>MSSAIKEVQGAPVKWVTNWTPEAIRGLVDQEKGLLD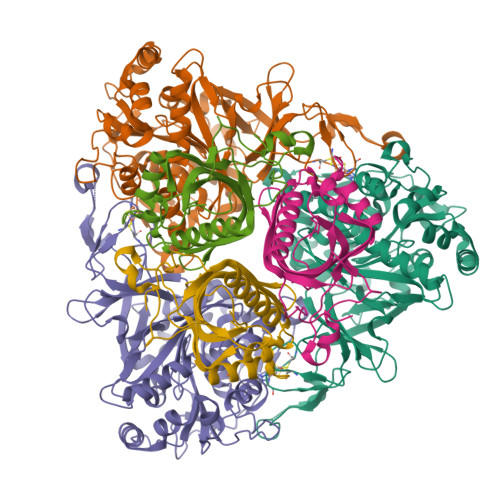PRIYADQSLYELELERVFGRSWLLLGHESHVPETGDFLATYMGEDPVVMVRQKDKSIKVFLNQCRHRGMRICRSDAGNAKAFTCSYHGWAYDIAGKLVNVPFEKEAFCDKKEGDCGFDKAEWGPLQARVATYKGLVFANWDVQAPDLETYLGDARPYMDVMLDRTPAGTVAIGGMQKWVIPCNWKFAAEQFCSDMYHAGTTTHLSGILAGIPPEMDLSQAQIPTKGNQFRAAWGGHGSGWYVDEPGSLLAVMGPKVTQYWTEGPAAELAEQRLGHTGMPVRRMVGQHMTIFPTCSFLPGINTIRTWHPRGPNEIEVWAFTLVDADAPAEIKEEYRRHNIRNFSAGGVFEQDDGENWVEIQKGLRGYKAKSQPLNAQMGLGRSQTGHPDFPGNVGYVYAEEAARGMYHHWMRMMSEPSWATLKP[4x];>[4x]MTNPSPHFFKTFEWPSKAAGLELQNEIEQFYYREAQLLDHRAYEAWFALLDKDIHYFMPLRTNRMIREGELEYSGDQDLAHFDETHETMYGRIRKVTSDVGWAENPPSRTRHLVSNVIVKETATPDTFEVNSAFILYRNRLERQVDIFAGERRDVLRRADNNLGFSIAKRTILLDASTLLSNNLSMFF>[2x]VLNSESLLRELRDALHEGGLTGSFLVRDLYTGEELGIDPDTELPTASLVKLPLALATLERIRLGEVDGAQQIEVAPGRITTPGPTGLSRFRHPARVAVDDLLYLSTSVSDGTASDALFEITPPAQVEQMVRE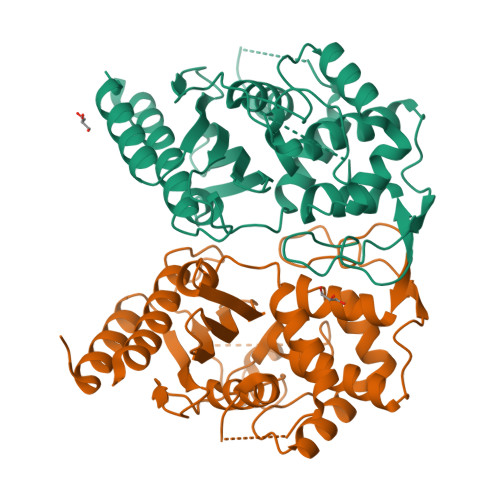WGFRDLTVRHSMRELSETPAERFESADAHLAHALAISAGTSGRGHRVPQLDVARANTGTARAFVDLLEALWAPVLTGPRPGRTSRALPPEPAARLRELMAANLLRHRLAPDFASDAATWSSKTGTLLNLRHEVGVVEHADGQVFAVAVLTESQVPADSQPGAEALMAQVARRLRDRLREWHHHHHH> MVTIVPYSHQYLKDICQLIQKDLSEPYSKYVYRYFVHQWPEFSFVALDNDRFIGAVICKQDVHRGTTLRGYIAMLAIVKEYRGQGIATKLTQASLDVMKNRGAQEIVLETEVDNEAAMSFYERLGFCRYKRLYRYYLNGTDAFRYILYPN;> MSVKESLSLLNSMQGNVKIGNVEPAKGNEGYVDNAGYVDCTKSYFEATKSLKEEQLVCDPKFTLLDSISAFEIMEPKMDSGIDYQPLRV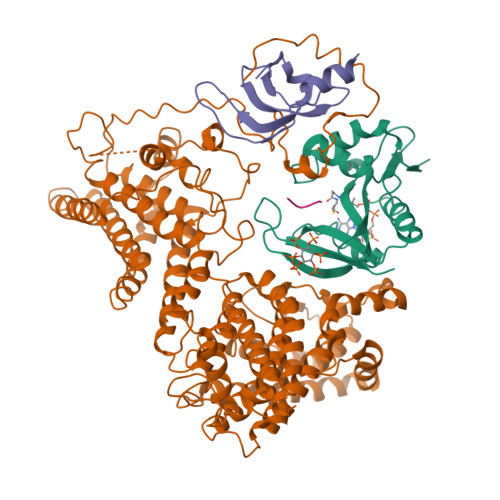DFSRDLSYLEILALMDLIVSAEKEWHYGSPLSESLLCSAHVFSICKSPISQVGDSGFSSGSGRNTTDIVLFPFVLAVIKCCDIVHREFLMGNLYDEEDISSFSYHMSFLQNYPIEKLNYLLQSSIEYLASEVIKFSAELRQIIEGILNRIQLRIGILRVYERSDIKTTIDALHLIKNLVPEIQNTVSVVDSSIKESILKQYWDFRVQAQLVATAPVRNIPPTGIEHSYQRILYFADDMLLILNSHTLASSLAVYQFCLDFTRLNRTPEPYVRSSLQALITANNAVNLRDQPTSYMLECIREFSGLPSNFYNPNTRTVIEKNSISSAYGPLVESLIAHSTNIMVDLVRICSHNPCRFRRNLINLLPEITVAHFEAEALDLKFVAKSLPSNGPFSSFIYHVKLNAIEHILLSSFEQKLHQPYQWPHFFAVLDHVFSIHQTHLELHGKDRNTPPMAKTFVTYLHRILNAIKETYSGYLLLTVLCMRLNIIKTPSFTLDEKIQESYYMAHYRPLINLRQPKPLLRSEADCIIKNLQNFSTDDLIIKSNEKFTAAKNSLINVIKSGFEQNEFINPYFLQTNYLKNLLCCCITNLVSLAILSKDHSANLKIVEIPGNPLPSLSRT;> MALHYFLQYDVQILCIALMFSIFRVCISTAIDFTSPKLDEFSLIMEMGEILLTSWLNRSVHIEIFDERKFIGKFLCTDREGAAILSNTTEYNKGFSRALGLVVIPGKHIKSFSVRA;> MLGP> SSQIRQNYSTEVEAAVNRLVNLYLRASYTYLSLGFYFDRDDVALEGVCHFFFELAFEKFEGAFRLLKMQNQRGGRALFQDLQKPSQDEWGTTLDAMKAAIVLEKSLNQALLDLHALGSAQADPHLCDFLESHFLDEEVKLIKKMGDHLTNIQRLVGSQAGLGEYLFERLTLKHD

As a scaffold for aromatic cluster design, we chose ferritin as a protein cage platform with a 12 nm outer diameter and an 8 nm inner cavity, composed of 24 subunits. To prove this concept through protein engineering, we focused on a two‐fold symmetric inter‐subunit interface of a recombinant horse spleen apo‐L ferritin (Fr) as a target region for mutagenesis. Herein, we present the construction of an aromatic cluster with an artificial molecular binding pocket at the two‐fold symmetric interface of ferritin and explore its ligand‐binding characteristics. We developed a system that uses ligand binding as a driving force to induce and propagate changes in the orientation of multiple aromatic side chains.

The resulting mutants were named Fr‐F2 (Fr‐E56F/R59F), Fr‐F4 (Fr‐R52F/E56F/R59F/E63F), and Fr‐F6 (Fr‐E53F/E56F/E57F/R59F/E60F/E63F), where i in Fr‐Fi represents the number of newly introduced Phe residues per ferritin monomer (upper). Within the vicinity of pocket F59, an intricate network of aromatic interactions is established, comprising three phenylalanine (Phe) residues (F52, F56, and F63) in Fr‐F4 and five Phe residues (F53, F56, F57, F60, and F63) in Fr‐F6. Analysis of the 2Fo‐Fc maps revealed electron densities corresponding to Nile Red (NR) at the two‐fold symmetric interfaces of NR•Fr‐F1, NR•Fr‐F2, NR•Fr‐F4, and NR•Fr‐F6, observed as overlapping densities due to the interface symmetry. NR was positioned between two F59 residues, forming π–π stacking interactions in an F59–NR–F59' configuration. In NR•Fr‐F4, a change in the χ1 angle of F56 was noted among the four introduced Phe residues, but no significant orientation changes were observed for the other Phe residues (F52, F59, F63). The quantum yield of Nile Red (NR) significantly increased from 0.50 in 100% methanol (MeOH) and 0.38 in a 50% MeOH‐water mixture to 0.88–0.95 upon encapsulation within Fr‐F1, Fr‐F2, Fr‐F4, and Fr‐F6. Furthermore, NR's fluorescence lifetime extended from 2.87 ns in organic solvent and 1.26 ns in aqueous‐organic mixture to 5.23–5.75 ns within these ferritin variants.>ATDYVALGDSYSSGVGAGSYDSSSGSCKRSTKSYPALWAASHTGTRFNFTACSGARTGDVLAKQLTPVNSGTDLVSITIGGNDAGFADTMTTCNLQGE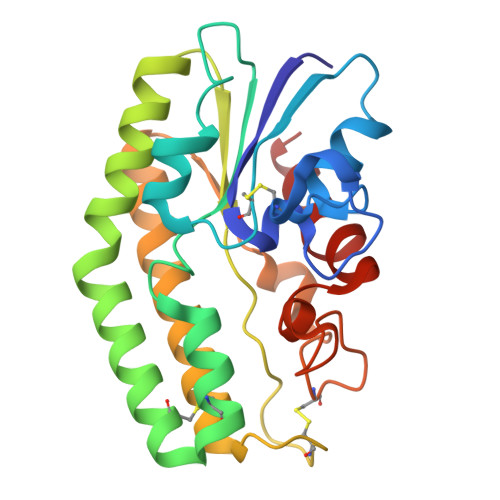SACLARIAKARAYIQQTLPAQLDQVYDAIDSRAPAAQVVVLGYPRFYKLGGSCAVGLSEKSRAAINAAADDINAVTAKRAADHGFAFGDVNTTFAGHELCSGAPWLHSVTLPVENSYHPTANGQSKGYLPVLNSAT[2x]> MLSLRQSIRFFKPATRTLCSSRYLLQQKPVVKTAQNLAEVNGPETLIGPGAKEGTVPTDLDQETGLARLELLGKLEGIDVFDTKPLDSSRKGTMKD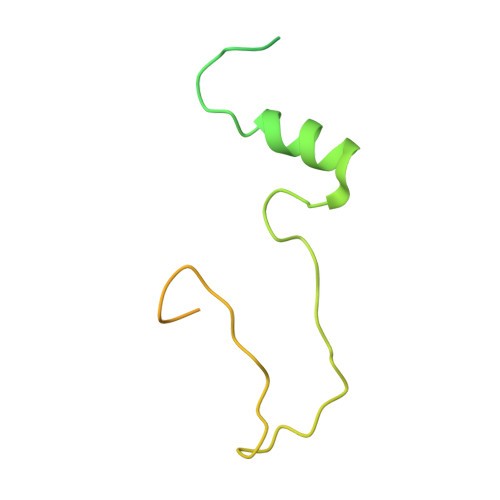PIIIESYDDYRYVGCTGSPAGSHTIMWLKPTVNEVARCWECGSVYKLNPVGVPNDDHHH Catalases (hydrogen-peroxide:hydrogen-peroxide oxido­reductases; EC 1.11.1.6) are redox enzymes that are responsible for the dismutation of hydrogen peroxide into water and molecular oxygen. The structures reveal a homotetrameric enzyme in which each of the four active sites consists of a pentacoordinated iron protoporphyrin IX prosthetic group with a tyrosin­ate axial ligand. The heme is deeply buried inside the protein, with a complex network of channels providing access to the exterior. We have previously shown that in addition to catalase activity, the catalase from S. thermophilum (CATPO) possesses a promiscuous phenolic oxidase activity in the absence of hydrogen peroxide.

We therefore generated a series of site-directed mutants around the putative 3TR/catechol binding pocket to further test this hypothesis. The residues Pro158, His246, Gln293, Ile313, Ile314, Glu316, Leu321 and Val536 surround the 3TR binding pocket and are structurally homologous to the residues that bind NADPH in the mammalian catalases. Specifically, the variants P158W, H246W, Q293W, I313F, I314F, E316F, E316H, L321A, V536A and V536W were constructed. The catechol oxidase activities of the H246W, I314F, L321A and V536W variants were noticeably reduced (50–92%) with respect to the wild-type enzyme, whereas the E316F, E316H, I313F and V536A variants of CATPO had little effect on the oxidase activity. A similar picture is seen for His246, which lies directly below and perpendicular to the 3TR ring in the CATPO–3TR complex.

>[4x]SPLAAYEVDDSTGYLTSDVGGPIQDQTSLKAGIRGPTLLEDFMFRQKIQHFDHERVPERAVHARGAGAHGTFTSYADWSNITAASFLNATGKQTPVFVRFSTVAGSRGSADTARDVHGFATRFYTDEGNFDIVGNNIPVFFIQDAIQFPDLIHSVKPRPDNEIPQAATAHDSAWDFFSQQPSTMHTLFWAMSGHGIPRSYRHMDGFGVHTFRFVKDDGSSKLIKWWFKSRQGKASLVWEEAQVLSGKNADFHRQDLWDAIESGNGPEWDVCVQIVDESQAQAFGFDLLDPTKIIPEEYAPLTKLGLLKLDRNPTNYFAETEQVMFQPGHIVRGIDFTEDPLLQGRLFSYLDTQLNRNGGPNFEQLPINMPRVPIHNNNRDGAGQMFIHRNKYPYTPNTLNSGYPRQANQNAGRGFFTAPGRTASGALVREVSPTFNDHWSQPRLFFNSLTPVEQQFLVNAMRFEISLVKSEEVKKNVLTQLNRVSHDVAVRVAAAIGLGAPDADDTYYHNNKTAGVSIVGSGPLPTIKTLRVGILATTSESSALDQAAQLRTRLEKDGLVVTVVAETLREGVDQTYSTADATGFDGVVVVDGAAALFASTASSPLFPTGRPLQIFVDAYRWGKPVGVCGGKSSEVLDAADVPEDGDGVYSEESVDMFVEEFEKGLATFRFTDRFALDS In order to unravel the molecular basis of the substrate and product specificity of NTMT2, we determine the X-ray crystal structures of NTMT2 in binary complex with SAM, as well as in ternary complex with SAH and an RCC1-derived peptide (SPKRIA). In addition, NTMT2 contains two auxiliary regions: an N-terminal α-lid (η1, α1–α2), and a β-lid (β6–β7) inserted between β5 and α8. These two lids cover the core domain that contributes to the substrate recognition. We also identify that N89 serves as a gatekeeper residue to control the entry of substrate into the active pocket.

To determine the molecular basis of different product specificities between NTMT2 and NTMT1, we solved crystal structures of the NTMT2-SAM binary complex and the NTMT2-SAH-SPKRIA peptide  ternary complex. The NTMT2-SAM binary complex subtly differs from the NTMT2-SAH-SPKRIA ternary complex in that the turn of the β-lid of the ternary complex is shifted closer to the catalytic core, which facilitates hydrogen bonding between substrate K3 and both D232 and D235 of NTMT2. The co-factor SAH/SAM in the ternary complex is nearly superimposable with that in the substrate-free binary complex. Based on sequence alignments, the N-terminal methyltransferases have a conserved DxGxGxGR motif located on the β1–α4 loop, which is involved in the SAH/SAM binding.

> GTSQVINGEMQFYARAKLFYQEVPATEEGMMGNFIELSSPDIQASQKFLRKFVGGPGRAGTDCALDCGSGIGRVSKHVLLPVFNSVELVDMMESFLLEAQNYLQVKGDKVESYHCYSLQEFTPPFRRYDVIWIQWVSGHLTDKDLLAFLSRCRDGLKENGIIILKDNVAREGCILDLSDSSVTRDMDILRSLIRKSGLVVLGQEKQDGFPEQCIPVWMFALH1-[3-(2-ethoxyethoxy)-5,5,8,8-tetramethyl-6,7-dihydronaphthalen-2-yl]-2-(trifluoromethyl)benzimidazole-5-carboxylic acid | C27 H31 F3 N2 O4 | 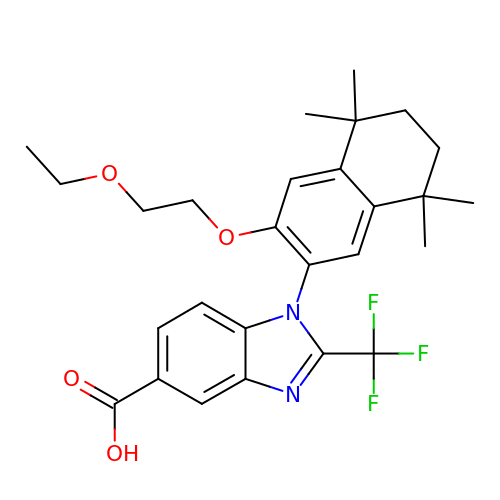FKCNXNPZSKIRIX-UHFFFAOYSA-N>[2x]VHINKGGRPRQHLLSLTRRAQKHRLRELKIQVKEFADKEEGGDVKAVCLTLFLLALRARNEHRQADELEAIMQGRGSGLQPAVCLAIRVNTFLSCSQYHKMYRTVKAITGRQIFQPLHALRNAEKVLLPGYHPFEWQPPLKNVSSRTDVGIIDGLSGLASSVDEYPVDTIAKRFRYDSALVSALMDMEEDILEGMRSQDLDDYLNGPFTVVVKESCDGMGDVSEKHGSGPAVPEKAVRFSFTVMRITIEHGSQNVKVFEEPKPNSELCCKPLCLMLADESDHETLTAILSPLIAEREAMKSSELTLEMGGIPRTFKFIFRGTGYDEKLVREVEGLEASGSVYICTLCDTTRLEASQNLVFHSITRSHAENLQRYEVWRSNPYHESVEELRDRVKGVSAKPFIETVPSIDALHCDIGNAAEFYKIFQLEIGEVYKHPNASKEERKRWQATLDKHLRKRMNLKPIMRMNGNFARKLMTQETVDAVCELIPSEERHEALRELMDLYLKMKPVWRSSCPAKECPESLCQYSFNSQRFAELLSTKFKYRYEGKITNYFHKTLAHVPEIIERDGSIGAWASEGNQSGNKLFRRF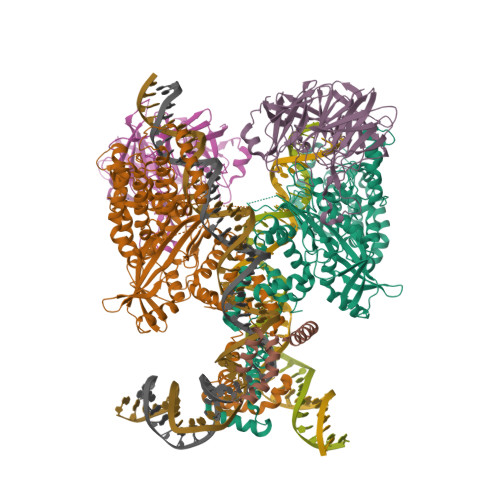RKMNARQSKCYEMEDVLKHHWLYTSKYLQKFMNAHNA;>MSLQMVTVGHNIALIQPGFSLMNFDGQVFFFGQKGWPKRSCPTGVFHFDIKQNHLKLKPAIFSKDSCYLPPLRYPATCSYKGSIDSDKHQYIIHGGKTPNNELSDKIYIMSVACKNNKKVTFRCTEKDLVGDVPEPRYGHSIDVVYSRGKSMGVLFGGRSYMPSTQRTTEKWNSVADCLPHVFLIDFEFGCATSYILPELQDGLSFHVSIARNDTVYILGGHSLASNIRPANLYRIRVDLPLGTPAVNCTVLPGGISVSSAILTQTNNDEFVIVGGYQLENQKRMVCSLVSLGDNTIEISEMETPDWTSDIKHSKIWFGSNMGNGTIFLGIPGDNKQAMSEAFYFYTLRCSEEDLSEDQ[2x];> MGKGDPKKPRGKMSSYAFFVQTCREEHKKKHPDASVNFSEFSKKCSERWKTMSAKEKGKFEDMAKADKARYEREMKTYIPPKGETKKKFKDPNAPKRPPSAFFLFCSEYRPKIKGEHPGLSIGDVAKKLGEMWNNTAADDKQPYEKKAAKLKEKYEKDIAAYR>[2x]MKESPKVVLLLTHSGDFFTIDRVAEAIEKKGATPFRLDTDKFPLEVQLTAQFNGKKSFYQLSYNHQSIDSEQVQSVWTRRIWQPELTGDLDPQFREVCVRESQTTLAGFWDSLRSARWLDNLAQIEKAKNKLLQLRLASEVGLIIPPTLVTNNPDAAREFFSQVQGRMVSKLLTAIARSMESPEFFLYTSRVKAED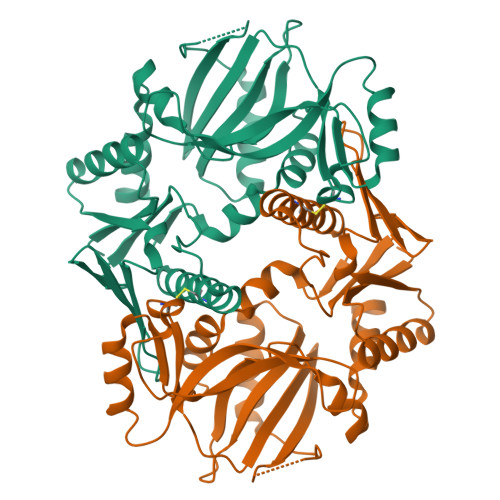LEEAESLRYCPMVFQAEIPKQLELRVVVVNGQTFVGALESSQYNNSAVDWRRPGIDPGAWQHHTLPDSLLQQLQIFMANLGLNFGAFDFILTPGGEYVFLEVNPGGEWGMLERDLDLPISQAIADFLVFGAAAHHHHHH>[2x]GSHPFDQAVVKDPTASYVDVKARRTFLQSGQLDDRLKAALPKEYDCTTEATPNPQQGEMVIPRRYLSGNHGPVNPDYEPVVTLYRDFEKISATLGNLYVATGKPVYATCLLNMLDKWAKADALLNYDPKSQSWYQVEWSAATAAFALSTMMAEPNVDTAQRERVVKWLNRVARHQTSFPGGDTSCCNNASYWRGQEATIIGVISKDDELFRWGLGRYVQA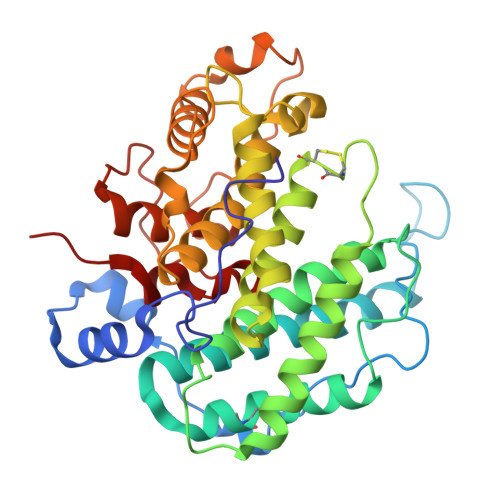MGLINEDGSFVHEMTRHEQSLHYQNYAMLPLTMIAETASRQGIDLYAYKENGRDIHSARKFVFAAVKNPDLIKKYASEPQDTRAFKPGRGDLNWIEYQRARFGFADELGFMTVPIFDPRTGGSGTLLAYKPQG> MSEENKPVEREEDTVRYEIVNNVAWVYYNRPTKRNAQSPKLNRQMLKVLTELEFRDDVGVLVLGGEGPAWCAGMDLKEYFRETEAEGLAGTRKAQREAYTWWERLRWYQKPTI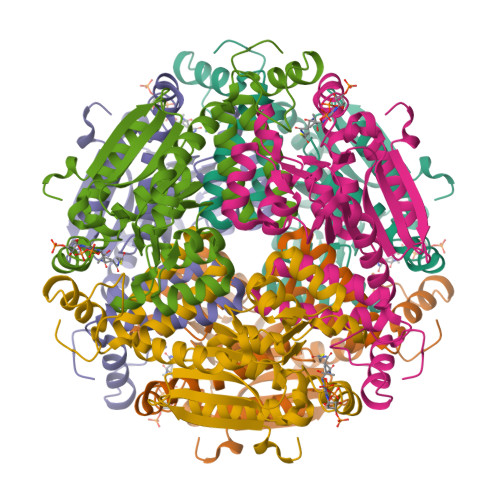AMVHGWCFGGAYGPLFACDLAFAADEAQFGLSEVNWGILPGGGATKVAVDLMPMRVAMYHAMMGENLSGQDAARYNLVNESMPADQLKARVKQVAETLIQKNWATVKYTKDAVRRVKEMTYDNAEDYLIRLQEGLNWFDKSDGRHVAMKQFLDDKTFKPGLGHYDKTKTEVLEHHHHHH>[11x]GSHM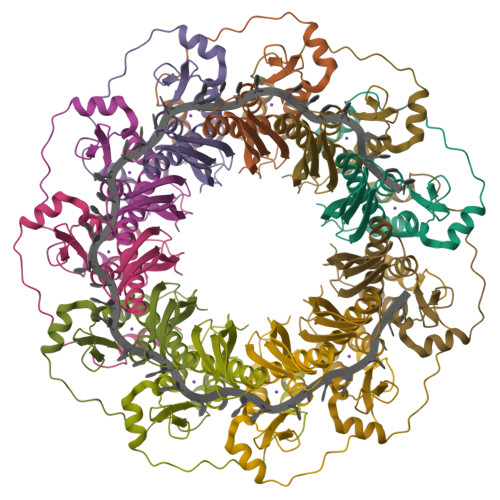SGTEEAILGGRDSHPAAGGGSVLCFGQCQYTAEEYQAIQKALRQRLGPEYISSRMAGGGQKVCYIEGHRVINLANEMFGYNGWAHSITQQNVDFVDLNNGAFYVGVCAFVRVQLKDGSYHEDVGYGVSEGLASKALSLEKARKEAVTDGLKRALRSFGNALGNCILDKDYLRSLNKLPRQLPLEVDLTKAKRQDLEPSVEEARYNSCRPNM>ETEAIDNGALREEAKGVFEAIPEKMTAIKQTEDNPEGVPLTAEKIELGKVLFFDPRMSSSGLISCQTCHNVGLGGVDGLPTSIGHGWQKGPRNAPTMLNAIFNAAQFWDGRAADLAEQAKGPVQAGVEMSNTPDQVVKTINSMPEYVEAFKAAFPEEADPVTFDNFAAAIEQFEATLITPNSAFDRFLAGDDAAMTDQEKRGLQAFMETGCTACHYGVNFGGQDYHPFGLIAKPGAEVLPAGDTGRFEVTRTTDDEYVFRAAPLRNVALTAPYFHSGVVWELAEAVKIMSSAQIGTELTDQQAEDITAFLGTLTGEQPVIDHPILPVRT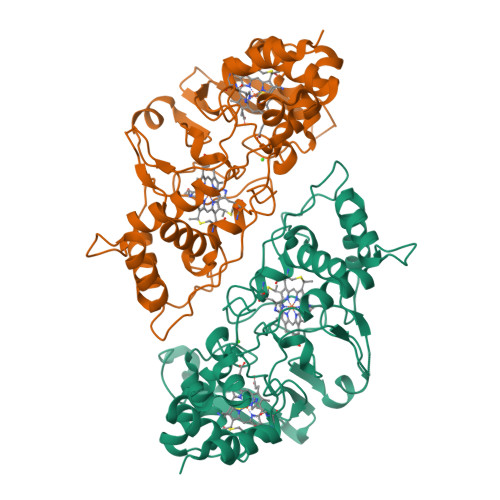GTTPLPTPM[4x]> GPMAIGLPSINISFKELATTVKERSARGIIAMVLKDAKALGLNEIHEKEDIPVDLSAENKEYINLALMGNVNTPNKLLVYVIEGEADIQTALDFLETKEFNYLCMPKAVEADKTAIKNW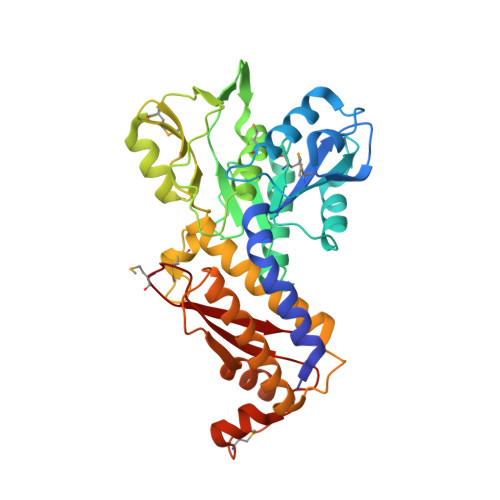IIKLRDIDKVKVKAVLGKVVGNHEGIINFTTEDVLVGEKKYSVDEFTSRVAGLIAGTPLSQSVTYTKLSDVVDIPKMTKVDAESKVNKGELILIKEAGAIRIARGVNSLTELTAEKGEMFQKIKIVDTLDIIHSDIRKVIIDDYIGKVTNSYDNKCLLIVAIKSYLEELEKSALIESDSTVEIDFEAQKSYLKSKGVDLSYMTLQEIKEANTGSKVFLKAKIKVLDAMEDIDLSIEI> 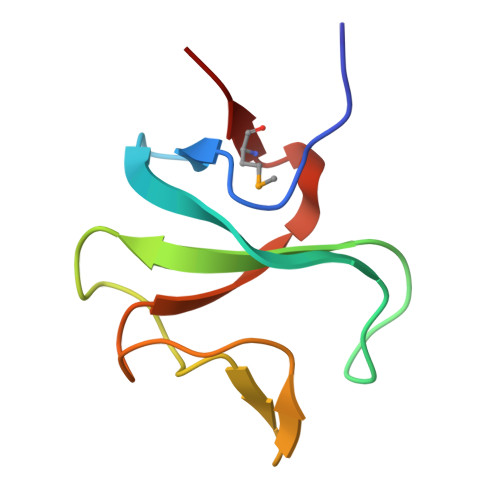GSDFRVGERVWVNGNKPGFIQFLGETQFAPGQWAGIVLDEPIGKNDGSVAGVRYFQCEPLKGIFTRPSKMTRKV> GPLGSMSGGFELQPRDGGPRVALAPGETVIGRGPLLGITDKRVSRRHAILEVAGGQL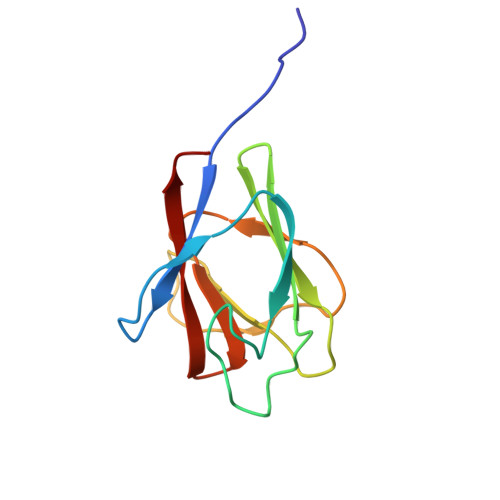RIKPIHTNPCFYQSSEKSQLLPLKPNLWCYLNPGDSFSMLVDKYIFRILSIPSA>GPEPDMISVFIGTWNMGSVPPPKNVTSWFTSKGLGKTLDEVTVTIPHDIYVFGTQENSVGDREWLDLLRGGLKELTDLDYRPIAMQSLWNIKVAVLVKPEHENRISHVSTSSVKTGIANTLGNKGAVGVSFMFNGTSFGFVNCHLTSGNEKTARRNQNYLDILRLLSLGDRQLNADDISDRFTHLFWFGDLNYRLDMDIQEILNYISRKEFEPLLRVDQLNLEREKHKVFLRFSEEEISFPPTYRYERGSRDTYAWHKQKPTGVRTNVPSWCDRILWKSYPETHIICNSYGCTDDIVTSDHSPVFGTFEVGVTSQFISKKGLSKTSDQAYIEFESIEAIVKTASRTKFFIEFYSTCLEEYKKSFENDAQSSDNINFLKVQWSSRQLPTLKPILADIEYLQDQHLLLTVKSMDGYESYGECVVALKSMIGSTAQQFLTFLSHRGEETGNIRGSMKVRVPTER[2x]

The two main enzymes responsible for PI(3,4,5)P3 degradation are the tumor suppressor phosphatase and tensin homolog (PTEN), which removes the 3-phosphate (3 P) and the SH2-containing inositol 5-phosphatase (SHIP), which dephosphorylates the 5 P to generate PI(3,4)P2. The SHIP Ptase domain belongs to a family of Mg2+-dependent inositol phosphatases with specificity for 5 P dephosphorylation of inositol rings. Here, we report the crystal structure of SHIP2 containing the 5-Ptase and a C2 domain (Ptase-C2), revealing that the two domains tightly associate via an extensive interface. Importantly, even in the absence of a localization effect, the C2 domain provides activating signals to the Ptase active site, resulting in a significant increase in catalytic turnover.

In order to disrupt the hydrophobic core of the domain interface we mutated F593 and L597 to aspartates (FLDD mutant). Crystal structures of Ptase-C2 FLDD confirm that few hydrophobic interactions remain intact between the Ptase and C2 domains. The FLDD mutations also disrupt interdomain hydrogen bonds between R649 and E862. When comparing the catalytic turnover of the FLDD mutants we find that the C2 domain no longer has a significant effect with either substrate, indicating that the FLDD mutations largely mimic the absence of the C2 domain. We note that the FLDD mutations increase intrinsic Ptase activity with PI(3,4,5)P3-diC8, but importantly the presence of the C2 does not cause any further change. The PS-mediated increase in activity on vesicles is maintained for the FLDD mutant, whereas as with soluble substrates, the increase in activity due to the C2 domain is abrogated by the interface mutations. Removing the C2 domain abolishes observed SHIP2 activity, whereas the FLDD mutations partially reduce activity of the wild-type protein.> PKR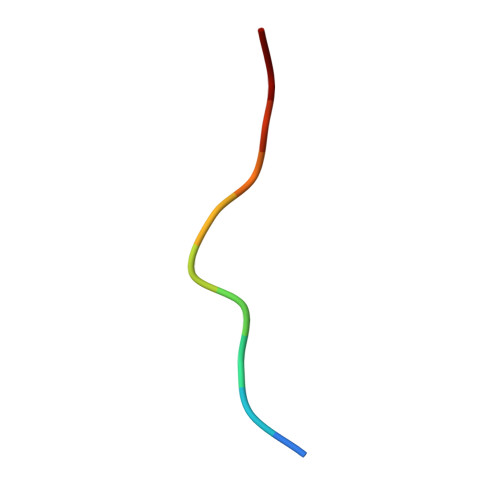PTTLNLF>MEPRPTAPSSGAPGLAGVGETPSAAALAAARVELPGTAVPSVPEDAAPASRDGGGVRDEGPAAAGDGLGRPLGPTPSQSRFQVDLVSENAGRAAAAAAAAAAAAAAAGAGAGAKQTPADGEASGESEPAKGSEEAKGRFRVNFVDPAASSSAEDSLSDAAGVGVDGPNVSFQNGGDTVLSEGSSLHSGGGGGSGHHQHYYYDTHTNTYYLRTFGHNTMDAVPRIDHYRHTAAQLGEKLLRPSLAELHDELEKEPFEDGFANGEESTPTRDAVVTYTAESKGVVKFGWINGVLVRCMLNIWGVMLFIRLSWIVGQAGIGLSVLVIMMATVVTTITGLSTSAIATNGFVRGGRAYYLISRSLGPEFGGAIGLIFAFANAVAVAMYVVGFAETVVELLKEHSILMIDEINDIRIIGAITVVILLGISVAGMEWEAKAQIVLLVILLLAIGDFVIGTFIPLESKKPKGFFGYKSEIFNENFGPDFREEETFFSVFAIFFPAATGILAGANISGDLADPQSAIPKGTLLAILITTLVYVGIAVSVGSCVVRDATGNVNDTIVTELTNCTSAACKLNFDFSSCESSPCSYGLMNNFQVMSMVSGFTPLISAGIFSATLSSALASLVSAPKIFQALCKDNIYPAFQMFAKGYGKNNEPLRGYILTFLIALGFILIAELNVIAPIISNFFLASYALINFSVFHASLAKSPGWRPAFKYYNMWISLLGAILCCIVMFVINWWAALLTYVIVLGLYIYVTYKKPDVNWGSSTQALTYLNALQHSIRLSGVEDHVKNFRPQCLVMTGAPNSRPALLHLVHDFTKNVGLMICGHVHMGPRRQAMKEMSIDQAKYQRWLIKNKMKAFYAPVHADDLREGAQYLMQAAGLGRMKPNTLVLGFKKDWLQADMRDVDMYINLFHDAFDIQYGVVVIRLKEGLDISHLQGQEELLSSQEKSPGTKDVVVSVEYSKKSDLDTSKPLSEKPITHKVEEEDGKTATQPLLKKESKGPIVPLNVADQKLLEASTQFQKKQGKNTIDVWWLFDDGGLTLLIPYLLTTKKKWKDCKIRVFIGGKINRIDHDRRAMATLLSKFRIDFSDIMVLGDINTKPKKENIIAFEEIIEPYRL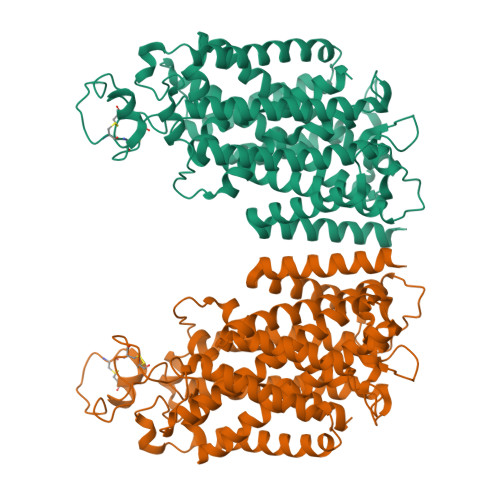HEDDKEQDIADKMKEDEPWRITDNELELYKTKTYRQIRLNELLKEHSSTANIIVMSLPVARKGAVSSALYMAWLEALSKDLPPILLVRGNHQSVLTFYS[2x]>FPKVATNIMRAWLFQHLTHPYPSEEQKKQLAQDTGLTILQ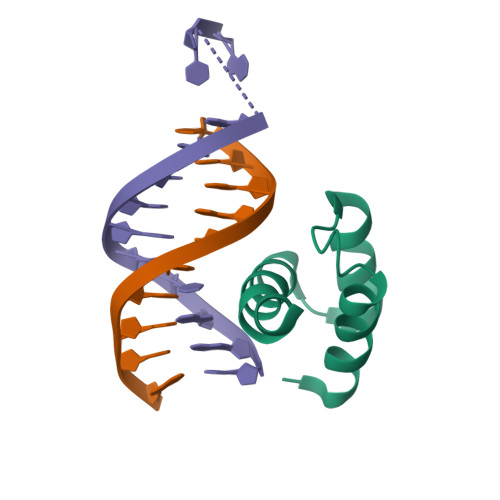VNNWFINARRRIVQPMIDQS[2x]> GHHHHHHHHHHSSGHIEGRHMKRMIALDGAQGEGGGQILRSALSLSMITGQPFTITSIRAGRAKPGLLRQHLTAVKAATEICGATVEGAELGSQRLLFRPGTVRGGDYRFAIGSAGSCTLVLQTVLPALWFADGPSRVEVSGGTDNPSAPPADFIRRVLEPLLAKIGIHQQTTLLRHGFYPAGGGVVATEVSPVASFNTLQLGERGNIVQMRGEVLLAGVPRHVAER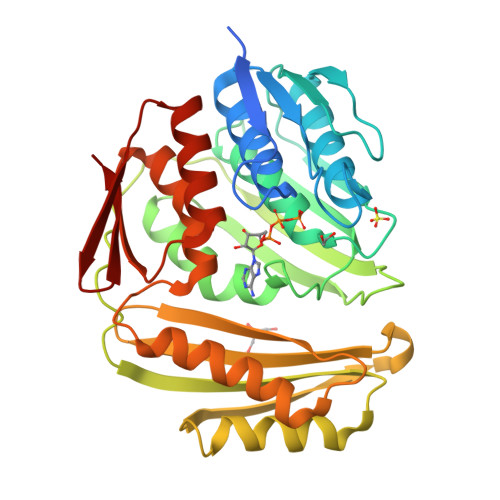EIATLAGSFSLHEQNIHNLPRDQGPGNTVSLEVESENITERFFVVGEKRVSAEVVAAQLVKEVKRYLASTAAVGEYLADQLVLPMALAGAGEFTVAHPSSNLLTNIAVVERFLPVRFSLIETDGVTRVSIE>MANKPTQPLFPLGLETSESSNIKGFNNSGTIEHSPGAVMTFPEDTEVTGLPSSVRYNPDSDEFEGYYENGGWLSLGGGGIRWETLPHAPSSNLLEGRGYLINNTTGTSTVVLPSPTRIGDSVTICDAYGKFATYPLTVSPSGNNLYGSTEDMAITTDNVSATFTWSGPEQGWVITSGVGLGQGRVYSREIFTQILASETSAVTLNTPPTIVDVYADGKRLAESKYSLDGNVITFSPSLPASTELQVIEYTPIQLGNGGGSGSSTITWVYNGGSAIGGETEITLDIVVDDVPAIDINGSRQYKNLGFTFDPLTSKITLAQELDAEDEVVVIINGTPHHHHHH[2x]

Bacteriophage (phage) vB_EcoM_CBA120, discovered by Kutter and colleagues, is a member of the recently defined Kuttervirus genus of contractile tailed phages belonging to the Ackermannviridae family. Each TSP recognizes a different lipopolysaccharide on the membrane of a different bacterial host. The 335 N-terminal residues of TSP4 promote the assembly of the TSP complex and anchor it to the tail baseplate.

TSP4-N335 crystals grown in KNa-tartrate solution diffracted to the highest resolution. Subsequently, the three resolved SeMet-TSP4-N335 domains were used as search models for molecular replacement with diffraction data from the wild-type protein crystals grown in KNa-tartrate. The resulting electron density map enabled tracing of the XD3 domains. TSP4-N335 associates into an elongated trimer, ~ 115 Å in length and ~ 65 Å at its widest region. A monomeric subunit comprises four domains; AD, XD1, XD2 and XD3. The XD2 and XD3 domains share the same threefold symmetry axis as the AD and XD1 domains such that three XD2 domains splay apart and do not interact with one another whereas the three XD3 domains pack together around the threefold symmetry axis. The separated XD2 modules lack continuous surface for binding a trimeric partner TSP, which is unlikely to represent the physiological structure. In contrast, the three TSP4 -N335 XD3 modules pack closely, with the adjacent N- and C-termini placed within a face perpendicular to the threefold symmetry axis. Consequently, the opposing face provides an uninterrupted trimeric surface where a partner TSP trimer can bind. The third linker connects the TSP4 XD2 and XD3 domains by a glycine-rich flexible long polypeptide (Thr250-Pro-Ile-Gln-Leu-Gly-Asn-Gly-Gly-Gly-Ser-Gly-Ser-Ser-Thr264) that is structurally disordered as manifested by the lack of associated interpretable electron density maps for both the wild-type and SeMet TSP4-N335 crystal structures.> LHPIIQIDRSFMLLILE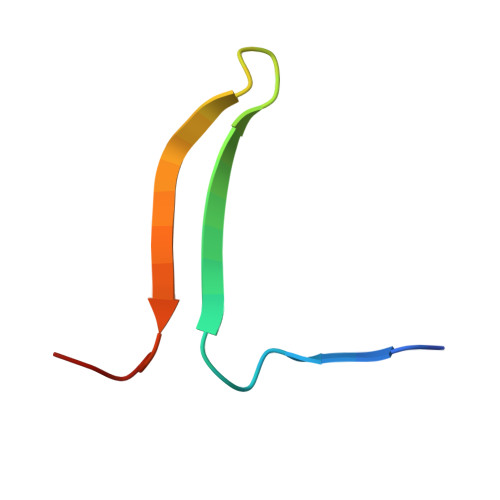RSTRSILFLGKVVNPTEA(5aS,12aS,13aS)-12,12-dimethyl-2,3,11,12,12a,13-hexahydro-1H,5H,6H-5a,13a-(epiminomethano)indolizino[7,6-b]carbazol-14-one | C21 H25 N3 O | 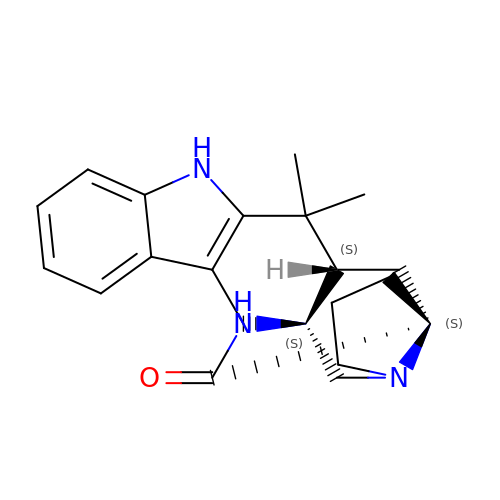LBTZXCFDJFHPMI-DQLDELGASA-N> MVPISPIETVPVKLKPGMDGPKVKQWPLTE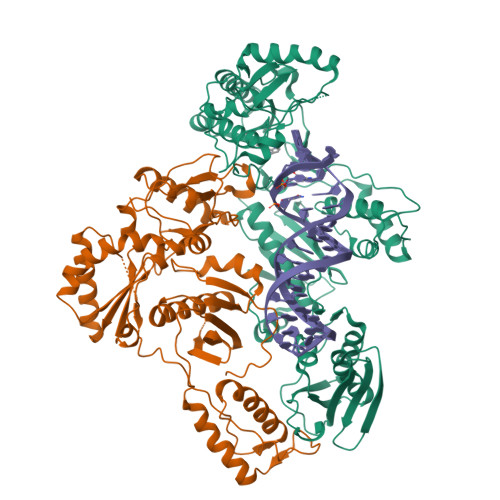EKIKALVEICTEMEKEGKISKIGPENPYNTPVFACKKKDSTKWRKLVDFRELNKRTQDFWEVQLGIPHPAGLKKKKSVTVLDVGDAYFSVPLDEDFRKYTAFTIPSINNETPGIRYQYNVLPQGWKGSPAIFQSSMTKILEPFKKQNPDIVIYQYMDDLYVGSDLEIGQHRTKIEELRQHLLRWGLTTPDKKHQKEPPFLWMGYELHPDKWTVQPIVLPEKDSWTVNDIQKLVGKLNWASQIYPGIKVRQLSKLLRGTKALTEVIPLTEEAELELAENREILKEPVHGVYYDPSKDLIAEIQKQGQGQWTYQIYQEPFKNLKTGKYARMRGAHTNDVKQLTEAVQKITTESIVIWGKTPKFKLPIQKETWETWWTEYWQATWIPEWEFVNTPPLVKLWYQLEKEPIVGAETFYVDGAANRETKLGKAGYVTNKGRQKVVPLTNTTNQKTELQAIYLALQDSGLEVNIVTNSQYALGIIQAQPDKSESELVNQIIEQLIKKEKVYLAWVPAHKGIGGNEQVDKLVSA;> PISPIETVPVKLKPGMDGPKVKQWPLTEEKIKALVEICTEMEKEGKISKIGPENPYNTPVFAIKKKDSTKWRKLVDFRELNKRTQDFWEVQLGIPHPAGLKKKKSVTVLDVGDAYFSVPLDEDFRKYTAFTIPSINNETPGIRYQYNVLPQGWKGSPAIFQSSMTKILEPFKKQNPDIVIYQYMDDLYVGSDLEIGQHRTKIEELRQHLLRWGLTTPDKKHQKEPPFLWMGYELHPDKWTVQPIVLPEKDSWTVNDIQKLVGKLNWASQIYPGIKVRQLSKLLRGTKALTEVIPLTEEAELELAENREILKEPVHGVYYDPSKDLIAEIQKQGQGQWTYQIYQEPFKNLKTGKYARMRGAHTNDVKQLTEAVQKITTESIVIWGKTPKFKLPIQKETWETWWTEYWQATWIPEWEFVNTPPLVKLWYQ>[4x]MHHHHHHMKDKIID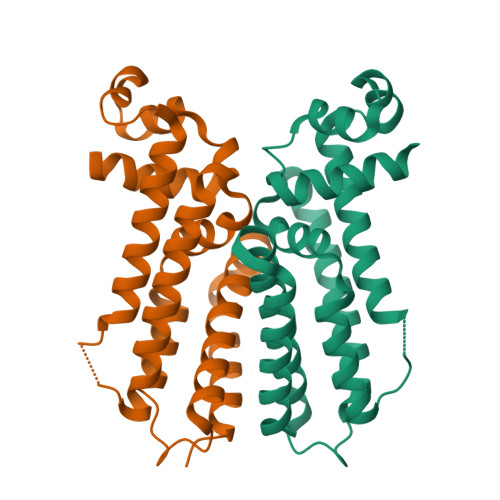NAITLFSEKGYDGTTLDDISKSVNIKKASLYYHYDNKEEIYRKSVENCFNYFIDFLLRNHDDNYSIDGLYQFLFKFIFDVDERYIKLYVQLSSAPEALNSEIKHHLQEINTTLHDELIKYYDPTHIALDKEDFINLILLFLETWYFRASFSQKFGIIEDSKNRFKDQVYSLLNVFLKK> PRRGAVAHANSIVQQLVSEGADISHTRNMLRNAMNGDAVAFSRVEQNIFRQHFPNMPMHGISRDSELAIELRG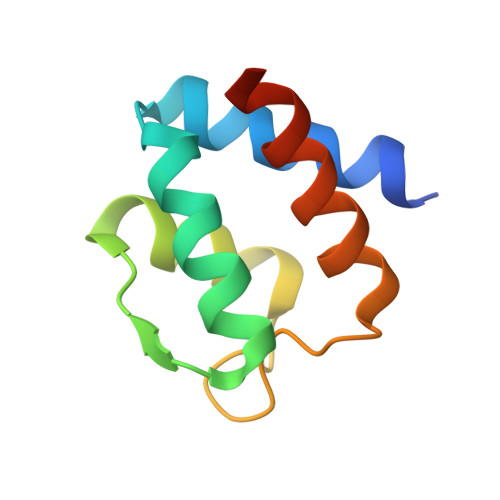ALRRAVHQQAAS>MGQSHTHDHHHDGYQAPPEDIALRVKALESLLIEKGLVDPAAMDLVVQTYEHKVGPRNGAKVVAKAWVDPAYKARLLADGTAGIAELGFSGVQGEDMV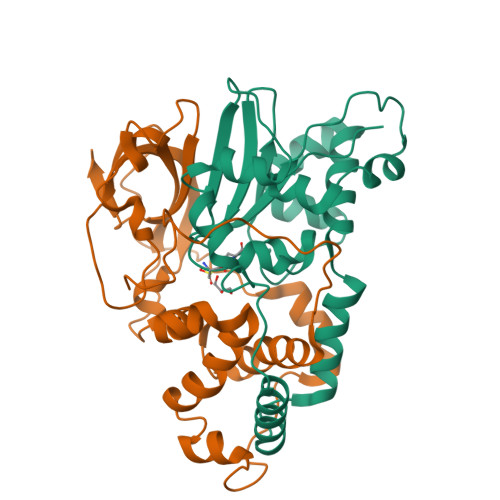ILENTPAVHNVFVCTLCSCYPWPTLGLPPAWYKAAPYRSRMVSDPRGVLAEFGLVIPANKEIRVWDTTAQLRYMVLPERPAGTEAYSEEQLAELVTRDSMIGTGLPTQPTPSH[4x];>MNGIHDTGGAHGYGPVYREPNEPVFRYDWEKTVMSLLPALLANGNFNLDEFRHSIERMGPAHYLEGTYYEHWLHVFENLLVEKGVLTATEVATGKAASGKTATPVLTPAIVDGLLSTGASAAREEGARARFAVGDKVRVLNKNPVGHTRMPRYTRGKVGTVVIDHGVFVTPDTAAHGKGEHPQHVYTVSFTSVELWGQDASSPKDTIRVDLWDDYLEPA[4x]> MATSGANGPGSATASASNPRKFSEKIALQKQRQAE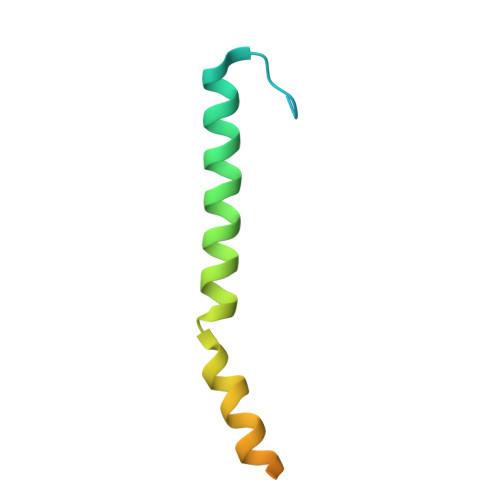ETAAFEEVMMDIGSTRLQAQKLRLAYTRSSHYGGSLPNVNQIGCG> GDPVEDIIHDALGSTARRAISSATNVESAANTTPSSHRLETGRVPALQAAETGATSNATDENMIETRCVVNRNGVLETTINHFFSRSGLVGVVNLTDGGTDTTGYVTWDIDIMGFVQLRRKCEMFTYMRFNAEFTFVTTTKNGEARPYMLQYMYVPPGAPKPTGRDAFQ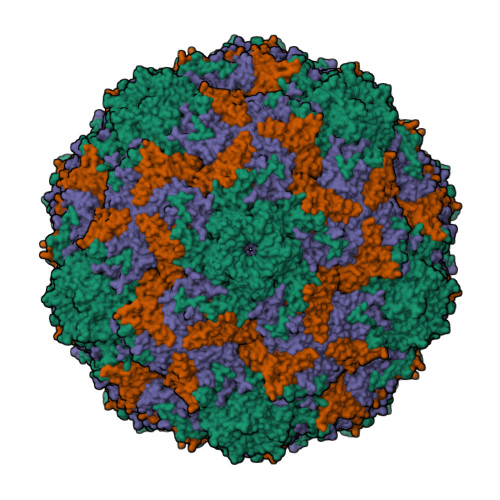WQTATNPSVFVKLTDPPAQVSVPFMSPASAYQWFYDGYPTFGQHPETSNTTYGLCPNNMMGTFAVRVVSREASQLKLQTRVYMKLKHVRAWVPRPIRSQPYLLKNFPNYDSSKITNSARDRSSIKQANM;> SPSVEACGYSDRVAQLTVGNSSITTQEAANIVLAYGEWPEYCPDTDATAVDKPTRPDVSVNRFYTLDSKMWQENSTGWYWKFPDVLNKTGVFGQNAQFHYLYRSGFCLHVQCNASKFHQGALLVAVIPEFVIAGRGSNTKPNEAPHPGFTTTFPGTTGATFHDPYVLDSGVPLSQALIYPHQWINLRTNNCATVIVPYINAVPFDSAINHSNFGLIVIPVSPLKYSSGATTAIPITITIAPLNSEFGGLRQAVSQ;> GIPAELRPGTNQFLTTDDDTAAPILPGFTPTPTIHIPGEVHSLLELCRVETILEVNNTTEATGLTRLLIPVSSQNKADELCAAFMVDPGRIGPWQSTLVGQICRYYTQWSGSLKVTFMFTGSFMATGKMLVAYSPPGSAQPANRETAMLGTHVIWDFGLQSSVSLVIPWISNTHFRTAKTGGNYDYYTAGVVTLWYQTNYVVPPETPGEAYIIAMGADLYKFTLKICKDTDEVTQQAVLQ> MDAAIRGNDVIFVLKTIGVPSACRQNEDPRFVEAFKCDELERYIENNPECTLFESLRDEEAYSIVRIFMDVDLDACLDEIDYLTAIQDFIIEVSNCVARFAFTECGAIHENVIKSMRSNFSLTKSTNRDKTSFHIIFLDTYTTMDTLIAMKRTLLELSRSSENPLTRSIDTAVYRRKTTLRVVGTRKNPNCDTIHVMQPPHDNIEDYLFTYVDMNNNSYYFSLQ

Helicase E5 is a multi-domain protein; its primer synthesis and DNA unwinding activity are required for genome uncoating and DNA replication of MPXV. MPXV E5 is encoded by the E5R gene, the mature protein is 785 amino acids (aa) in length. MPXV E5 can be divided into 6 domains: the AEP domain, the ZnD domain (Zinc-binding domain), the D5N domain (a domain associated with D5-type helicases), the Linker, the SF3 Helicase domain, and the C-Tail. MPXV E5 belongs to the SF3 helicase superfamily, which normally forms hexamer and unwinds DNA with 3′- to 5′ polarity.

In addition to the AEP domain of MPXV E5, we also performed crystallization study for the AEP domain of VACV D5 and solved one structure at 1.4-Å resolution. Similar to E5 AEP, one PPi was captured in the D5 AEP structure. As revealed by structural superposition, the overall folding of E5 and D5 AEP domains are virtually identical; the RMSD value between the two domains is only 0.2 Å. These observations indicated that the folding and catalytic activity of the AEP domains are highly conserved in MPXV E5, VACV D5, and the helicases from other orthopoxvirus viruses. Identical structures indicated that the overall folding and catalytic activity of the AEP domains are conserved in MPXV E5, VACV D5, and, most likely, in all other poxviruses members.> AQPDIKFASKEYGVTIGESRIIYPLDAAGVMVSVKNTQDYPVLIQSRIYDENKEKESEDPFVVTPPLFRLDAKQQNSLRIAQAGGVFPRDKESLKWLCVKGIPPKDEDIWVDDATNKQKFNPDKDVGVFVQFAINNCIKLLVRPNELKGTPIQFAENLSWKVDGGKLIAENPSPFYMNIGELTFGGK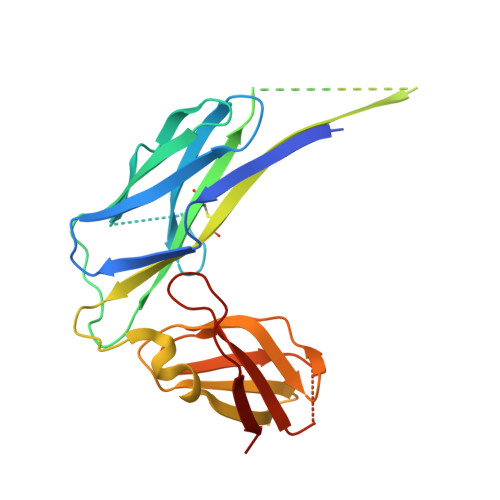SIPSHYIPPKSTWAFDLPKGLAGARNVSWRIINDQGGLDRLYSKNVTL> DA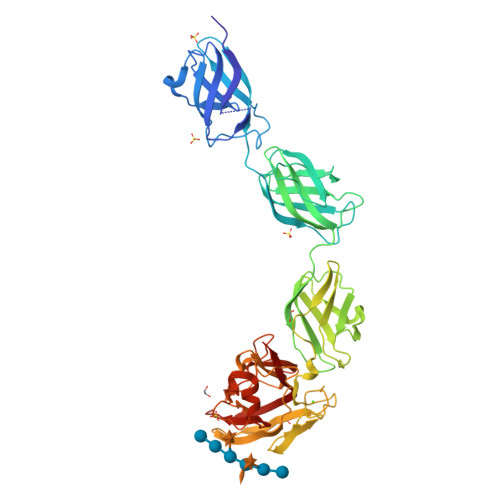IPVIHYIRVTDPAKADSTFTDVNPGTMIVVVGEHLGGTQKVYINDQEVSFNRNYVTSTSIILTVPNELELTGQNPELKGEIRIETEHGVAAYNMHVLSPAPYITRISATYPIKPGDQMTVIGGNFYEVQAVYLSTEQPAKDGTRPVDVQEITNYEVNNKYSQITLTAPANLLEEGYLVVECYTSSAVTEFKKNGPKPVVTAVSSTMPVVGSTVTITGQNFIEVSRVNINAEFDIPVGDITTSNTFDEISFVLPQAPTQSGHISVTAIGGTVESAEIFYPLENVILNYDGIGSHVWGDCSFVVADGSSAPYVSNGTCLGITGTVSASNYWWKQSYSNAQWVNTSIIPGNIPIDDLKLQFECFVKEVFTGPVFQIAMCENFDAALNGYVPVSSFTGKTETGKWMQCSVSLSSVVADATYQDFLNRNSTHIGVYATNPGSSQATIEVYFDNFRIVRK>[4x]MANDTPFSALWQRLLTRGWQPVEASTVDDWIKRVGDGVILLSSDPRRTPEVSDNPVMIAELLREFPQFDWQVAVADLEQSEAIGDRFNVRRFPATLVFTDGKLRGALSGIHPWA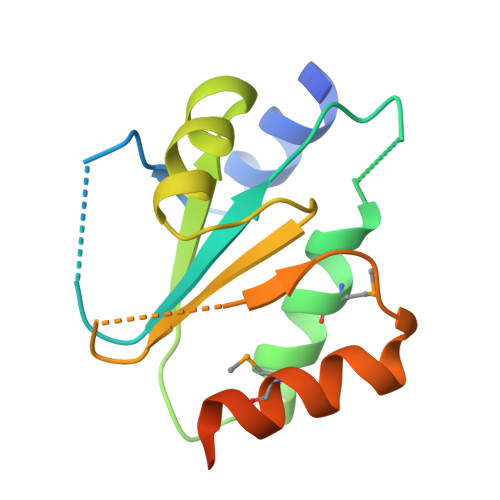ELLTLMRSIVDTPAAQETVQLEHHHHHH> GIQGLAKLIADVAPSAIRENDIKSYFGRKVAIDASMSIYQFLIAVRQGGDVLQNEEGETTSHLMGMFYRTIRMMENGIKPVYVFDGKPPQLKSGELAKRSERRAEAEKQLQQAQAAGAEQEVEKFTKRLVKVTKQHNDECKHLLSLMGIPYLDAPSEAEASCAALVKAGKVYAAATEDMDCLTFGSPVLMRHLTASEAKKLPI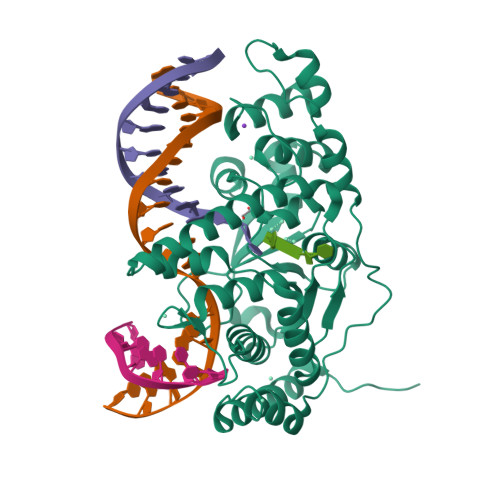QEFHLSRILQELGLNQEQFVDLCILLGSNYCESIRGIGPKRAVDLIQKHKSIEEIVRRLDPNKYPVPENWLHKEAHQLFLEPEVLDPESVELKWSEPNEEELIKFMCGEKQFSEERIRSGVKRLSKSRQGSTLEVLFQ>MSTPNVLTNVAVSHSGEVDSLLIEKFNGKVREQYLKGENLLSHFQVETVTGTNTVSNKYLGETEIQVLAPGQSPAATPTKADKNQVVIDTTVIARNTVAMLHDVQGDIDSLKPKIAVNQAKQLKRLEDEMVVQQLMLGGISNTKAQRTNPRVPGHGFSINVNITADTAETSPQYLAAAIEYALEQQLEQEVDISDLVILMPWKFFNALRDMDRIVDRSYTLADESTVQGFALKSFNVPVVPSNRFPKFSQGAAHHKLSNADNGFRYDTTAPMAGAVAVIFSMDALLVGRTIELTGDIFWEKKEK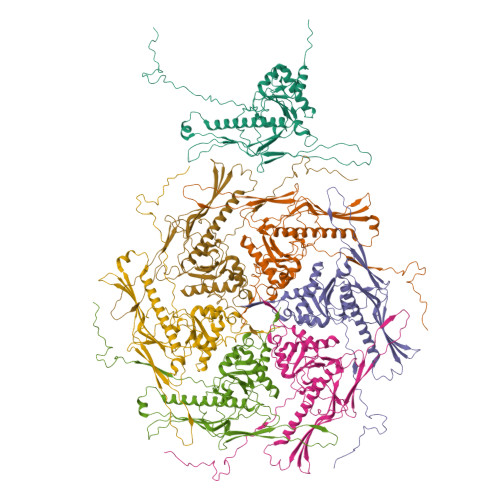TFYIDTYLAEGAIPDRWEAVSVVTTARNATTGDPDGTGADDTVVTKRANRKVILTKAVS[7x]2-(3-methoxypropyl)-3-oxo-2,3-dihydro-1H-isoindole-4-carboxamide | C13 H16 N2 O3 | 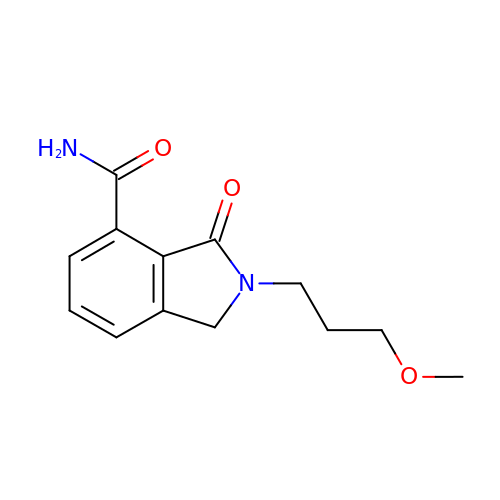VARCSQSOWLMGTH-UHFFFAOYSA-N ethyl benzylcarbamate | C10 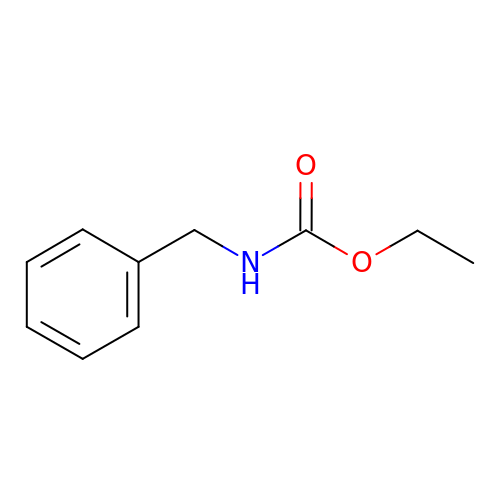H13 N O2 | XSXLCQLOFRENHC-UHFFFAOYSA-N> ASVHGTTYELLRRQGIDTVFGNPGSNELPFLKDFPEDFRYILALQEACVVGIADGYAQASRKPAFINLHSAAGTGNAMGALSNAWNSHSPLIVTAGQQTRAMIGVEALLTNVDAANLPRPLVKWSYEPASAAEVPHAMSRAIHMASMAPQGPVYLSVPYDDWDKDADPQSHHLFDRHVSSSVRLNDQDLDILVKALNSASNPAIVLGPDVDAANANADCVMLAERLKAPVWVAPSAPRCPFPTRHPCFRGLMPAGIAAISQLLEGHDVVLVIGAPVFRYHQYDPGQYLKPGTRLISVTCDPLEAARAPMGDAIVADIGAMASALANLVE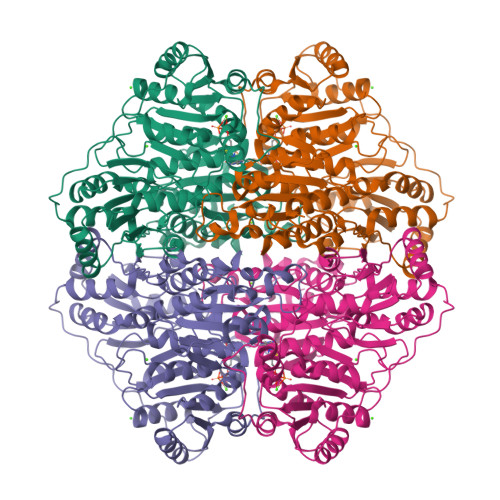ESSRQLPTAAPEPAKVDQDAGRLHPETVFDTLNDMAPENAIYLNESTSTTAQMWQRLNMRNPGSYYFCAAGGLGFALPAAIGVQLAEPERQVIAVIGDGSANYSISALWTAAQYNIPTIFVIMNNGTYGALRWFAGVLEAENVPGLDVPGIDFRALAKGYGVQALKADNLEQLKGSLQEALSAKGPVLIEVSTVSPVK> GSEGCVSNLMVCNLAYSGKLEELKESILADKSLATRTDQDSRTALHWACSAGHTEIVEFLLQLGVPVNDKDDAGWSPLHIAASAGRDEIVKALLGKGAQVNAVNQNGCTPLHYAASKNRHE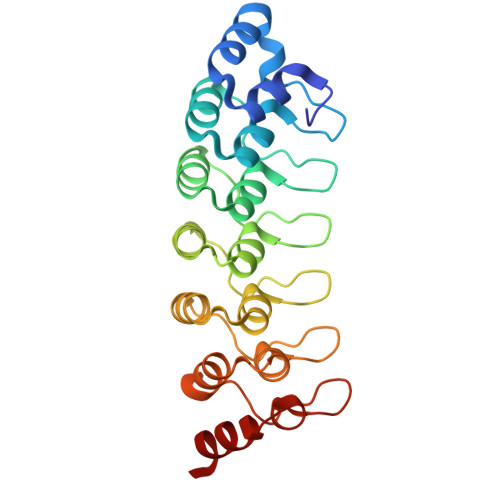IAVMLLEGGANPDAKDHYEATAMHRAAAKGNLKMIHILLYYKASTNIQDTEGNTPLHLACDEERVEEAKLLVSQGASIYIENKEEKTPLQVAKGGLGLILKRMVEG> RSMEDENVKKFIKEFEDTKIMPVRKGTKTTRTEKFYLVFTEWVKLLQRVENNDVITTVFIKQLVEKGVISDTDNLLTFVKSSLELSVSSFKESDPTDEVFIAIDALGSLIIKLLILQDFKDDTRRDYINAIFSVIVLVFAKDHSQEGTTFNERPYFRLFSNILYEWATIRTHNFVRIS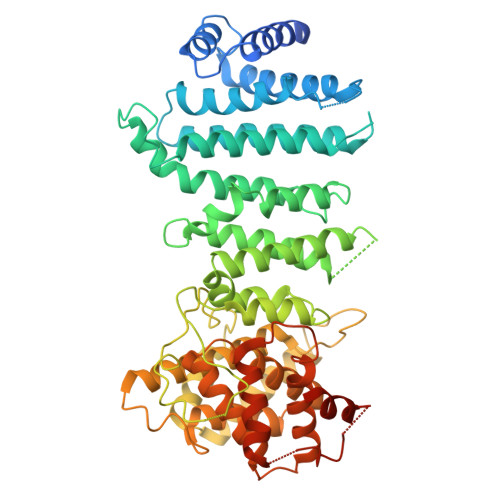DSSTRQELIEFDSVFYNTFSGYLHALQPFAFPGFSFAWVTLLSHRMLLPIMLRLPNKIGWEKLMLLIIDLFKFLDQYTSKHAVSDAVSVVYKGTLRIILGISNDMPSFLIENHYELMNNLPPTYFQLKNVILSAIPKNMTVPNPYDVDLNMEDIPACKELPEVFFDPVIDLHSLKKPVDNYLRIPSNSLLRTILSAIYKDTYDIKKGVGYDFLSVDSKLIRAIVLHVGIEAGIEYKRTSSNAVFNTKSSYYTLLFNLIQNGSIEMKYQIILSIVEQLRYPNIHTYWFSFVLMNMFKSDEWNDQKLEVQEIILRNFLKRIIVNKPHTWGVSVFFTQLINNNDINLLDLPFVQSVPEIKLILQQLVKYSKKYTTSEQDDQ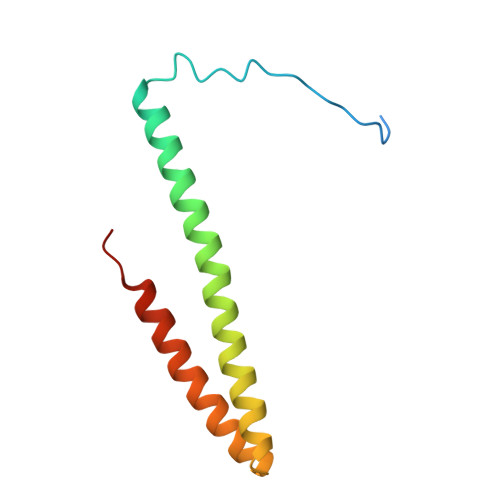> GSASSPVQSGFNNGTISNYMYFERRPDLLTKGTQDKAAAVKLKIENFYQSSVKYAIERNERRVELETELTSHNWSEERKSRQLSSLGKKESQFLRLRRTRLSLED> ARQNPGLA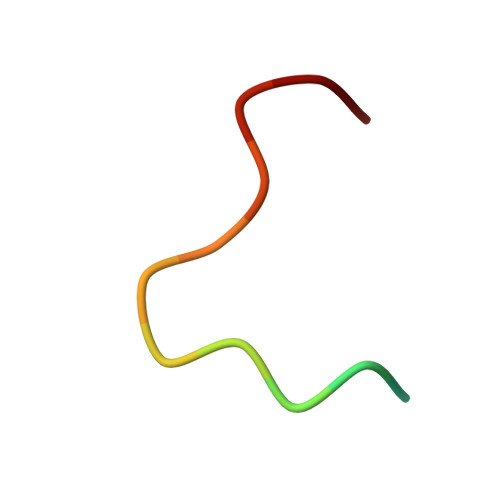YGNPYS> SQNLTCNSNDLKALEGFMRGLESSIDGWKWNESSSFSSNCCDWVGISCKSSVSLGLDDVNESGRVVELELGRRKLSGKLSESVAKLDQLKVLNLTHNSLSGSIAASLLNLSNLEVLDLSSNDFSGLFPSLINLPSLRVLNVYENSF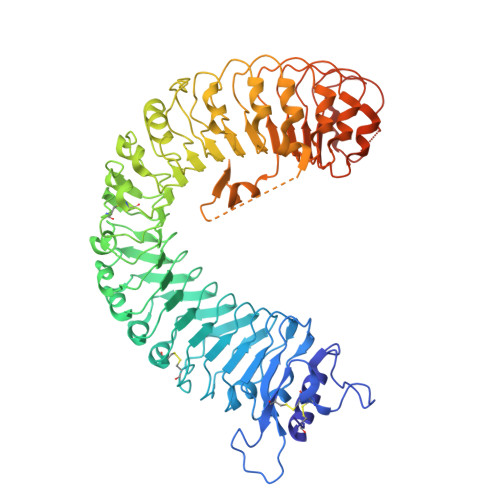HGLIPASLCNNLPRIREIDLAMNYFDGSIPVGIGNCSSVEYLGLASNNLSGSIPQELFQLSNLSVLALQNNRLSGALSSKLGKLSNLGRLDISSNKFSGKIPDVFLELNKLWYFSAQSNLFNGEMPRSLSNSRSISLLSLRNNTLSGQIYLNCSAMTNLTSLDLASNSFSGSIPSNLPNCLRLKTINFAKIKFIAQIPESFKNFQSLTSLSFSNSSIQNISSALEILQHCQNLKTLVLTLNFQKEELPSVPSLQFKNLKVLIIASCQLRGTVPQWLSNSPSLQLLDLSWNQLSGTIPPWLGSLNSLFYLDLSNNTFIGEIPHSLTSLQSLVSKENAVEEPSPDFPFFKKKNTNAGGLQYNQPSSFPPMIDLSYNSLNGSIWPEFGDLRQLHVLNLKNNNLSGNIPANLSGMTSLEVLDLSHNNLSGNIPPSLVKLSFLSTFSVAYNKLSGPIPTGVQFQTFPNSSFEGNQGLCGEHASPCHITDQSPHGSHHHHHH> SKFLDRFRYAKQKGETFADGHGQLLNTNRDWEDGYRQRWQHDKIVRSTHGVNCTGSCSWKIYVKNGLVTWETQQTDYPRTRPDLPNHEPRGCPRGASYSWYLYSANRLKYPMMRKRLMKMWREAKALHSDPVEAWASIIEDADKAKSFKQARGRGGFVRSSWQEVNELIAASNVYTIKNYGPDRVAGFSPIPAMSMVSYASGARYLSLIGGTCLSFYDWYCDLPPASPQTWGEQTDVPESADWYNSSYIIAWGSNVPQTRTPDAHFFTEVRYKGTKTVAVTPDYAEIAKLCDLWLAP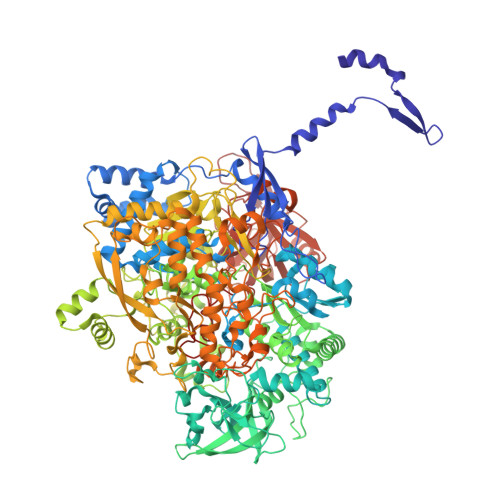KQGTDAAMALAMGHVMLREFHLDNPSQYFTDYVRRYTDMPMLVMLEERDGYYAAGRMLRAADLVAALGQENNPEWKTVAFNTNGEMVAPNGSIGFRWGEKGKWNLEQRDGKTGEETELQLSLLGSQDEIAEVGFPYFGGDGTEHFNKVELENVLLHKLPVKRLQLADGSTALVTTVYDLTLANYGLERGLNDVNCATSYDDVKAYTPAWAEQITGVSRSQIIRIAREFADNADKTHGRSMIIVGAGLNHWYHLDMNYRGLINMLIFCGCVGQSGGGWAHYVGQEKLRPQTGWQPLAFALDWQRPARHMNSTSYFYNHSSQWRYETVTAEELLSPMADKSRYTGHLIDFNVRAERMGWLPSAPQLGTNPLTIAGEAEKAGMNPVDYTVKSLKEGSIRFAAEQPENGKNHPRNLFIWRSNLLGSSGKGHEFMLKYLLGTEHGIQGKDLGQQGGVKPEEVDWQDNGLEGKLDLVVTLDFRLSSTCLYSDIILPTATWYEKDDMNTSDMHPFIHPLSAAVDPAWEAKSDWEIYKAIAKKFSEVCVGHLGKETDIVTLPIQHDSAAELAQPLDVKDWKKGECDLIPGKTAPHIMVVERDYPATYERFTSIGPLMEKIGNGGKGIAWNTQSEMDLLRKLNYTKAEGPAKGQPMLNTAIDAAEMILTLAPETNGQVAVKAWAALSEFTGRDHTHLALNKEDEKIRFRDIQAQPRKIISSPTWSGLEDEHVSYNAGYTNVHELIPWRTLSGRQQLYQDHQWMRDFGESLLVYRPPIDTRSVKEVIGQKSNGNQEKALNFLTPHQKWGIHSTYSDNLLMLTLGRGGPVVWLSEADAKDLGIADNDWIEVFNSNGALTARAVVSQRVPAGMTMMYHAQERIVNLPGSEITQQRGGIHNSVTRITPKPTHMIGGYAHLAYGFNYYGTVGSNRDEFVVVRKMKNIDWLDGEGNDQVQES>[2x]SPNYDKWEMERTDITMKHKLGGGQYGEVYEGVWKKYSLTVAVKTLKEDTMEVEEFLKEAAVMKEIKHPNLVQLLGVCTREPPFYIITEFMTYGNLLDYLRECNRQEVNAVVLLYMATQISSAMEYLEKKNFIHRDLAARNCLVGENHLVKVADFGLSRLMTGDTYTAHAGAKFPIKWTAPESLAYNKFSIKSDVWAFGVLLWEIATYGMSPYPGI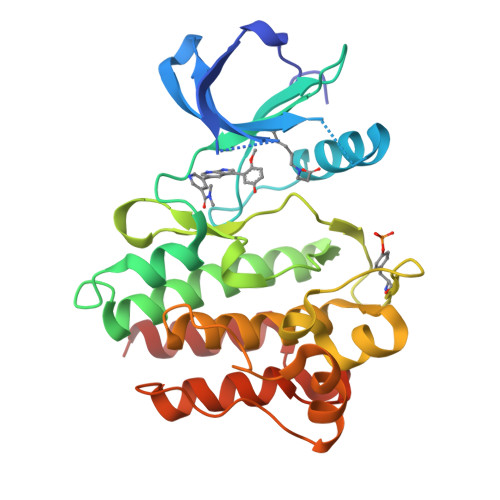DLSQVYELLEKDYRMERPEGCPEKVYELMRACWQWNPSDRPSFAEIHQAFETMFQES> MSKLQISNTCPDKYRTKQEGVEYPTAKKITYYSKVTETERKMNVILPVGYDENKKYPVVYYLHGLMSYEDSMLEDDSTLAIPTNLLKEGRAKEMIIVLPDVYAPKPGTAVTPDFNPEYYKGYDNFINELIEVIMPYMEEHYSILTGRENTALCGFSMGARTSLYIGYMRSDLIGYVGAFAPAPGITPGEDSFSGKHEGLISEDEFRAEIQPIVSLIDCGTNDSVVGQFPKSYHEILTRNNQEHIWFEVPGADHDWNAISA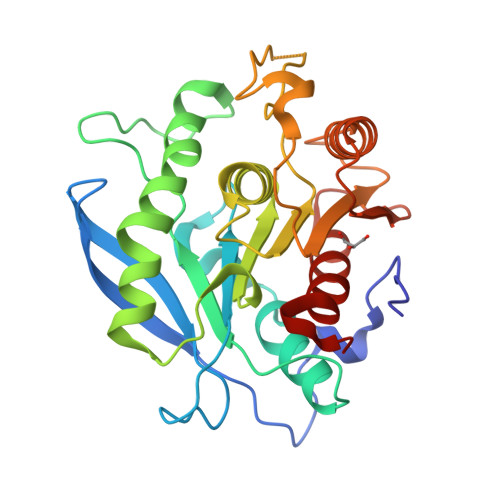GFYNFIQTTFGALNN>MSAIALYLEINKLRLKIDEPMQLAIWPQLFPLLCDEHQSVQLNTDVLINFMMHVARKSQNTILNNNAAIASQYAAGNADVVAAPASAQPTPRPVINLFARANAAAPAQPSEELINMRRYRNAARKLIHHYSLNSTSSTEYKISDVVMTMIFLLRSEKYHSLFKLLETTFDDYTCRPQMTQVQTDTLLDAVRSLLEMPSTTIDLTTVDIMRSSFARCFNSPIMRYAKIVLLQNVALQRDKRTTLEELLIERGEKIQMLQPQQYINSGTEIPFCDDAEFLNRLLKHIDPYPLSRMYYNAANTMFYTTMENYAVSNCKFNIEDYNNIFKVMENIRKHSNKNSNDQDELNIYLGVQSSNAKRKKY[2x];>MKRIKCNKVRTVTEIVNSDEKIQKTYELAEFDLKNLSSLESYETLKIKLALSKYMAMLSTLEMTQPLLEIFRNKADTRQIAAVVFSTLAFIHNRFHPLVTNFTNKMEFVVTETNDTSIPGEPILFTENEGVLLCSVDRPSIVKMLSREFDTEALVNFENDNCNVRIAKTFGASKRKNTTRSDDYESNKQPNYDMDLSDFSITEVEATQYLTLLLTVEHAYLHYYIFKNYGVFEYCKSLTDHSLFTNKLRSTMSTKTSNLLLSKFKFTIEDFDKINSNSVTSGFNIYNFNK[2x]

Baculovirus Autographa californica multiple nucleopolyhedrovirus (AcMNPV) has been widely used as a bioinsecticide and a protein expression vector. The DNA genome, along with the baculovirus basic DNA-binding protein P6.9 protein, is encapsulated by an enveloped, rod-shaped nucleocapsid; the major capsid protein VP39 and some additional minor proteins are known to comprise the nucleocapsid. Here, we show a 3.2 Å resolution structure of helical cylindrical body of the AcMNPV nucleocapsid, composed of VP39, as well as 4.3 Å resolution structures of both the head and the base of the nucleocapsid composed of over 100 protein subunits. Surprisingly, the C14 symmetric base had nearly identical features to that of the apical head, except for that in the central regions. Both the head and base could be further segmented into three parts: an outer shell, an inner layer and a central region.

Unique to the base, the plug occupies the innermost position and essentially seals one end of the capsid. In the base there is a “plug” that sits in the center-most portion sealing of the nucleocapsid; further analyses revealed that the plug density has C7 symmetry. Like the inner layer, each asymmetric unit of the plug is primarily composed of two copies of AC101 (AC101-3 and AC101-4) and two copies of AC144 (AC144-3 and AC144-4), though they arranged with C7 symmetry rather than C14 symmetry found in the inner layer. The interactions among the AC101 dimers, as well as between AC101 and AC144, are almost identical to those described in the inner layer. However, the long helix (Glu27-Leu61) of AC144-3 is bent near residue Leu39, resulting in the long helix being broken into two helices: helix 1 (Ala29-Ser38) and helix 2 (Leu39-Thr60), and helix 2 is rotated ~60° compared to that of AC144-1, allowing the N-terminal β-sheet to interact with AC101-3 and AC144-4 in the same manner seen in the inner layer, and thus anchoring AC101-3 to AC144-4. The rotation of helix 2 forces AC144-4 to rotate and point toward the C7 axis, effectively sealing the base domain. Interactions between the inner layer and the plug, primarily through several hydrogen bonds, take place at the interface between AC101-1 in the inner layer and AC144-3 in plug. These interactions allow two neighboring AC101 dimers in the inner layer to “clamp” one AC101-AC144 complex in the plug. Hence, the AC101 dimers in the inner layer link both the outer shell and plug together, and thus stabilize the base.> GPTIYHAKDAVQATKPDMRKPRLVVFVVGETARADHVSFNGYERDTFPQLAKIDGVTNFSNVTSCGTSTAYSVPCMFSYLGADEYDVDTAKYQENVLDTLDRLGVSILWRDNNSDSKGVMDKLPKAQFADYKSATNNAICNTNPYNECRDVGMLVGLDDFVAANNGKDMLIMLHQMGNHGPAYFKRYDEKFAKFTPVCEGNELAKCEHQSLINAYDNALLATDDFIAQSIQWLQTHSNAYDVSMLYVSDHGESLGENGVYLHGMPNAFAPKEQRSVPAFFWTDKQTGITPMATDTVLTHDAITPTLLKLFDVTADKVKDRTAFIR

MCR-1 confers resistance by modifying the colistin target, catalyzing transfer of phosphoethanolamine (PEA) onto the glucosamine saccharide of lipid A in the bacterial outer membrane. Bacterial lipooligosaccharide PEA-transferases such as MCR-1 are organised into two domains: an N-terminal inner membrane-bound domain predicted to contain 5 transmembrane α-helices and a soluble, periplasmic domain containing the putative catalytic centre. Here we present two crystal structures of the soluble, catalytic domain of MCR-1, revealing this to be a zinc metalloprotein containing three intramolecular disulphide bonds. The two structures are essentially identical (RMSD 0.37 Å over 311 Cα atoms) and reveal an overall α-β-α fold, containing three intramolecular disulphide bonds, typical of alkaline phosphatase or sulphatase enzymes, with the N-terminus indicating the likely position of the five transmembrane helices.

To facilitate such studies, we engineered MCR-1 to lack the five transmembrane helices, generating a construct containing residues 219–541 (MCR1ΔTM) which was purified and crystallised. Phases calculated from datasets collected at or near the zinc X-ray absorption edge ultimately yielded structures for two different crystal forms in the space groups P41212 (1.75 Å resolution) and P21 (1.55 Å resolution). However, the two crystal forms differ in zinc content, with the P21 structure containing one zinc ion (Zn1), coordinated by Asp465, His466, Glu246 and Thr285 in a tetrahedral geometry, while the P41212 structure contains density for an additional, also tetrahedral, zinc site (Zn2) coordinated by His395, His478, a water molecule (Wat1) and Glu300 from a symmetry related molecule. Whilst our structures unambiguously identify a zinc site (Zn1) in MCR-1 adjacent to the essential Thr285, the Zn2 site in the P41212 crystal form involves crystallographic contacts and may not be relevant in solution. This possibility is further supported by another recently released crystal structure of the MCR-1 catalytic domain with phospho-Thr285 (PDB 5K4P20) that was crystallised from conditions of high zinc concentration contains zinc ions in the Zn1 site and at a number of additional positions, of which none is directly equivalent to the Zn2 site identified here. However, less complete conservation is evident when comparing the putative Zn2 sites- while the Zn2 ligands His395 and His478, and the adjacent Glu468, are also well conserved between MCR-1, LptA and EptC, these positions vary in less closely related family members such as choline sulphatase suggesting that an intact Zn2 site is not a prerequisite for activity in all such enzymes.> MRKKSLTIFSDGTLLRRENTLY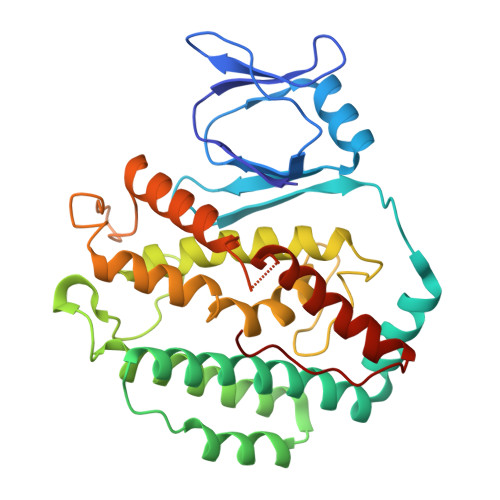FENVNGRKPLAIEGIYDIYIYGHVNITSQALHYIAQKGILIHFFNHYGYYDGTFYPRETLLSGDLIIKQAEHYLDKNKRLFLAKSFVVGGAKNMEKNLKNWGISSDFSNHLKELQGAKKVTEIMNVEGRIRQEYYARWDESLPGEFRIGKRTRRPPKNEMNALISFLNSRLYATMISEIYNTQLAPTISYLHEPSERRFSLALDLSEIFKPIIADRIANRLVKKGIIKKDHFREDLNGVLLTDEGMKIVTKAYNQELEKTVKHPKLGKGVTRRRLIRLEAYKIIKHLVGVEEYSPLVAWF The Notch signalling pathway is conserved across all metazoan species and plays key roles in many aspects of cell biology including cell‐fate determination, stem cell maintenance, immune system activation and angiogenesis in humans (Guruharsha et al, 2012; Bray, 2016). Aberrant Notch signalling results in a number of inherited and acquired disorders, including various cancers, and it is therefore a key target for therapeutic intervention (Hansson et al, 2004; Groth & Fortini, 2012). Both the Notch receptors and the ligands are single‐pass type I transmembrane proteins, and direct protein–protein contact between adjacent cells initiates an intracellular signalling pathway. All of the Notch ligands have a modular extracellular architecture consisting of an N‐terminal C2 domain (formerly known as the MNNL domain), a Delta/Serrate/Lag‐2 (DSL) domain, and either 16 (Jagged1/Jagged2), 8 (Delta‐like1/Delta‐like4) or 7 (Delta‐like3) EGF repeats. Binding of a Notch ligand to EGF11‐12 of a Notch receptor results in a series of proteolytic cleavages, with the final intra‐membrane cleavage by gamma secretase, causing the release of the intracellular domain of Notch (NICD) from the plasma membrane.

Here, we present the first structures of Jagged2 (N‐EGF2 and N‐EGF3), which has only 58% sequence identity with human Jagged1 (N‐EGF3), together with the longest known structure of a Delta‐like4 ligand (human Delta‐like4 N‐EGF3). We expressed and solved the structures of various N‐terminal fragments of both human Delta‐like4 and Jagged2. These fragments include the N‐terminal C2 lipid‐binding domain, the receptor‐binding DSL domain, and two (“N‐EGF2”) or three (“N‐EGF3”) adjacent EGF domains. Two crystal forms of Jagged2 (N‐EGF2) (green) and one crystal form of Jagged2 (N‐EGF3) (dark green) were solved, including a total of seven crystallographically independent copies of N‐EGF2, and 1 copy of N‐EGF3 (N.b. not all of EGF3 is visible in the electron density). All of these copies have been superposed on each other by alignment of the DSL domain, showing some flexibility in the hinge region between the C2 and DSL domains, and further flexibility in the hinge regions between the EGF domains. However, the angle between adjacent domains can vary subtly, resulting in the ligand structures appearing to fall into two groups, one group including Jagged1, Delta‐like1 and some structures of Jagged2, and the other including Delta‐like4, and some structures of Jagged2. The observation that Jagged2 is split across the two groups suggests that there is some flexibility between adjacent domains of the Notch ligands and that all may be able to adopt these different conformations. The Jagged1 and Jagged2 C2 domains bind calcium ions (shown in red), whereas Delta‐like4 and Delta‐like1 do not; the aspartates involved in calcium binding are not conserved in Delta‐like4 and Delta‐like1. Both Jagged1 and Jagged2 contain N‐glycosylation sites in the loop between strands 5 and 6.

> MGYFELQLSALRNVNGELLSGACCDGDGRTTRAGGCGHDECDTYVRVCLKEYQAKVTPTGPCSYGHGATPVLGGNSFYLPPAGAAGDRARARARAGGDQDPGLVVIPFQFAWPRSFTLIVEAWDWDNDTTPNEELLIERVSHAGMINPEDRWKSLHFSGHVAHLELQIRVRCDENYYSATCNKFCRPRNDFFGHYTCDQYGNKACMDGWMGKECKEAVCKQGCNLLHGGCTVPGECRCSYGWQGRFCDECVPYPGCVHGSCVEPWQCNCETNWGGLLCDKDLNYCGSHHPCTNGGTCINAEPDQYRCTCPDGYSGRNCEKAEGSHHHHHHHH>MKIQMRNKKVLSFLTLTAIVSQALVYPVYAQTSTSNHSNKKKEIVNEDILPNNGLMGYYFTDEHFKDLKLMAPIKDGNLKFEEKKVDKLLDKDKSDVKSIRWTGRIIPSKDGEYTLSTDRDDVLMQVNTESTISNTLKVNMKKGKEYKVRIELQDKNLGSIDNLSSPNLYWELDGMKKIIPEENLFLRDYSNIEKDDPFIPNNNFFDPKLMSDWEDEDLDTDNDNIPDSYERNGYTIKDLIAVKWEDSFAEQGYKKYVSNYLESNTAGDPYTDYEKASGSFDKAIKTEARDPLVAAYPIVGVGMEKLIISTNEHASTDQGKTVSRATTNSKTESNTAGVSVNVGYQNGFTANVTTNYSHTTDNSTAVQDSNGESWNTGLSINKGESAYINANVRYYNTGTAPMYKVTPTTNLVLDGDTLSTIKAQENQIGNNLSPGDTYPKKGLSPLALNTMDQFSSRLIPINYDQLKKLDAGKQIKLETTQVSGNFGTKNSSGQIVTEGNSWSDYISQIDSISASIILDTENESYERRVTAKNLQDPEDKTPELTIGEAIEKAFGATKKDGLLYFNDIPIDESCVELIFDDNTANKIKDSLKTLSDKKIYNVKLERGMNILIKTPTYFTNFDDYNNYPSTWSNVNTTNQDGLQGSANKLNGETKIKIPMSELKPYKRYVFSGYSKDPLTSNSIIVKIKAKEEKTDYLVPEQGYTKFSYEFETTEKDSSNIEITLIGSGTTYLDNLSITELNSTPEILDEPEVKIPTDQEIMDAHKIYFADLNFNPSTGNTYINGMYFAPTQTNKEALDYIQKYRVEATLQYSGFKDIGTKDKEMRNYLGDPNQPKTNYVNLRSYFTGGENIMTYKKLRIYAITPDDRELLVLSVD[2x];> YSEKVCNTTYKAPIERPEDFLKDKEKAKEWERKEAERIEQKLERSEKEALESYKKDSVEISKYSQTRNYFYDYQIEANSREKEYKELRNAISKNKIDKPMYVYYFESPEKFAFNKVIRTENQNEISLEKFNEFKETIQNKLFKQDGFKDISLYEPGKGDEKPTPLLMHLKLPRNTGMLPYTNTNNVSTLIEQGYSIKIDKIVRIVIDGKHYIKAEASVVSSLDFKDDVSKGDSWGKANYNDWSNKLTPNELADVNDYMRGGYTAINNYLISNGPVNNPNPELDSKITNIENALKREPIPTNLTVYRRSGPQEFGLTLTSPEYDFNKLENIDAFKSKWEGQALSYPNFISTSIGSVNMSAFAKRKIVLRITIPKGSPGAYLSAIPGYAGEYEVLLNHGSKFKINKIDSYKDGTITKLIVDATLIP

CDT is a member of the Iota family of protein toxins which also consists of two homologous toxins produced by Clostridium perfringens (the Iota toxin) and Clostridium spiroforme (C. spiroforme Transferase, CST). All three Iota toxin family members are assembled from two polypeptide chains termed the “A” subunit (CDTa, Ia, and CSTa) and “B”, subunit (CDTb, Ib, and CSTb). All three B subunits are presumed to contain five domains that are involved in regulation (D1), oligomerization (D2 and D3), and host recognition (D3’ and D4). Once proteolyzed, the mature form of CDTb forms a large heptameric, soluble structure referred to as the prepore which binds one molecule of CDTa to generate the toxic moiety, CDT.

During classification, we noted a population of the CDTb dimeric assembly intermediate bound to CDTa. Despite a significant number of particles observed in this complex, the three-dimensional reconstruction was limited to modest resolution (4.57 Å) due to issues arising from preferred orientation. Nonetheless, we have successfully assembled a pseudoatomic model of this interaction. The interface formed between CDTa and the CDTb dimer is facilitated by interactions with both chains of CDTb (buried surface areas of ~241 Å2 and ~122 Å2 were observed for Chains A and B, respectively). Though we note the resolution of the map hindered the assignment of residues at the interface, the CDTb dimer is confirmed to adopt a prepore-like configuration as observed in the apo structure (RMSD of 0.657 Å) and interacts with CDTa through a binding mode that is similar to that previously described (RMSD of 2.203 Å). Moreover, our data indicate that assembly intermediates can form interactions with CDTa, suggesting the enzymatic component spontaneously associates with the intermediates that form during assembly.> MKTRSQITCASLALLIAGSSLLYTTQTLIVKAEPTQSVSSSVQTSTQRDRNSVKQAVRDTLQLGFPGILAKTSEGGKTWSYAAGVANLSSKKPMKTDFRFRIGSVTKTFTATVVLQLAEENRLNLDDSIEKWLPGVIQGNGYDDKQITIRQLLNHTSGIAEYTRSKSFDLMDTKKSYRAEELVKMGISMPPDFAPGKSWSYSNTGYVLLGILIETVTGNSYAEEIENRIIEPLEL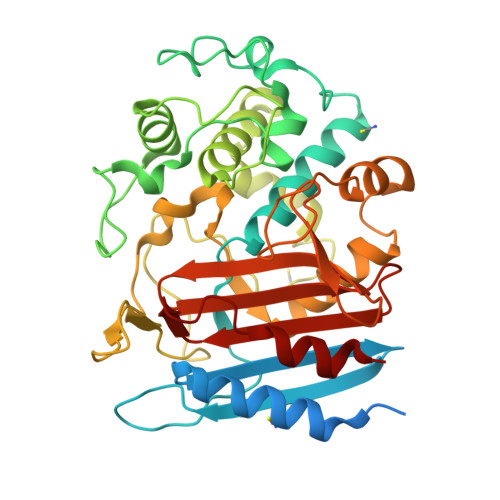SNTFLPGNSSVIPGTKHARGYIQLDGASEPKDVTYYNPSMGSSAGDMISTADDLNKFFSYLLGGKLLKEQQLKQMLTTVPTGEAALGRYGLGIYETKLPNGVSIWGHGGSIPGFVTFAGGTLGGKHTLAVNLNSLNAESPDPFKNILLAEFSK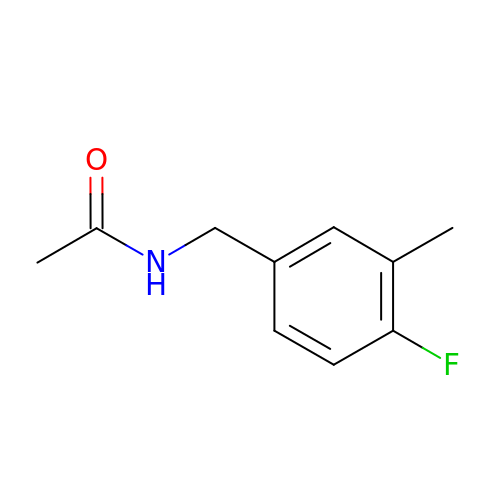N-[(4-fluoro-3-methylphenyl)methyl]acetamide | C10 H12 F N O | GEEDCVIVOYJQIC-UHFFFAOYSA-N> MTWGRAVILEAMRRYLQQRRAMEPWEDPAGISHLEIQKLMYFANEADPDLALDFTPGRYGPYSERVRHLLQGMEGAFTVGLGDGTARVLANQPISLTTKGTDAITDYLATDAAADRVSAAVDTVLRVIEGFEGPYGVELLAST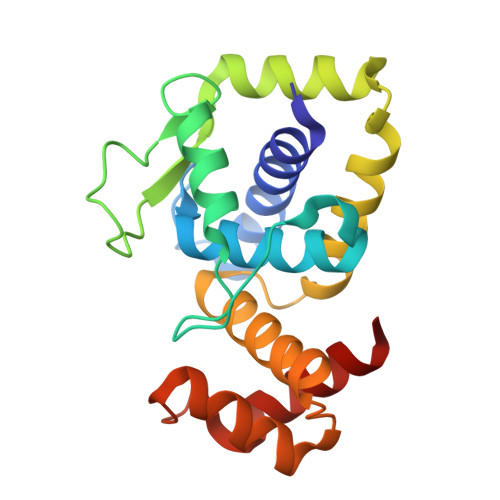HWVATREGAKEPATAAAAVRKWTKRKGRIYSDDRIGVALDRILMTA>DTSSQIKHASAVVSAPKDIAVAIGYMPEKYKAPWIIAMGVNLRAKRIIAEAEKYGVPIMRNVPLAHQLLDEGKELKFIPETTYEAVGEIL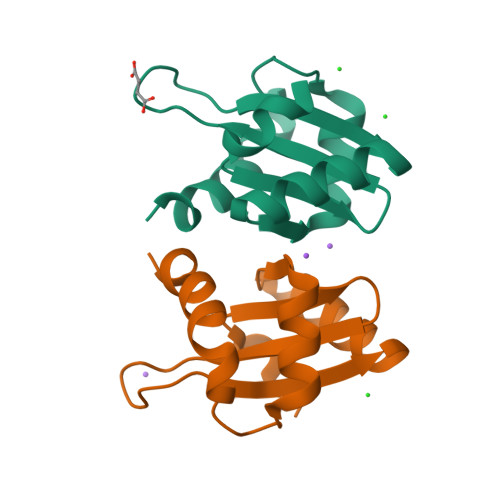LYITSLN[2x]>[2x]MEKVREIVREGIRVGNEDPRRIIHAFKVGLALVLVSSFYYYQPFGPFTDYFGINAMWAVMTVVVVFEFSVGATLGKGLNRGVATLVAGGLGIGAHQLARLSGATVEPILLVMLVFVQAALSTFVRFFPWVKTKFDYGILIFILTFALISLSGFRDEEIMDLAESRLSTVVIGGVSCILISIFVCPVWAGQDLHSLLASNFDTLSHFLQDFGDEYFEAREKGDYKVVEKRKKNLERYKSVLDSKSDEEALANYAEWEPPHGQFRFRHPWKQYVAVGALLRQCAYRIDALNSYINSDFQIPVDIKKKLETPLRRMSSESGNSMKEMSISLKQMIKSSSSDIHVSNSQAACKSLSTLLKSGILNDVEPLQMI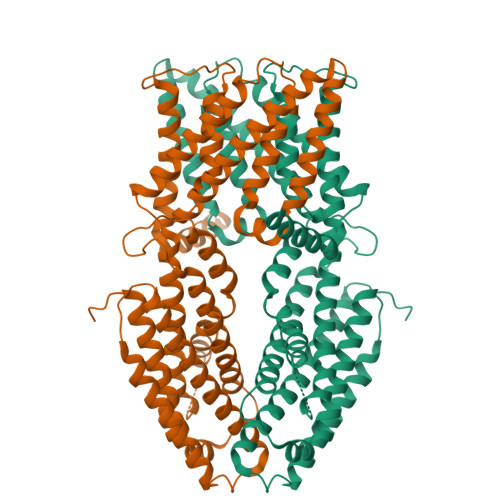SLMTTVSMLIDIVNLTEKISESVHELASAARFKNKMRPTVLYEKSDSGSIGRAMPIDSHEDHHVVTVLHDVDNDRSNNVDDSRGGSSQDSCHHVAIKIVDDNSNHEKHEDGEIHVHTLSNGHLQLEGGSSGGWSHPQFEK> GSTIQIPYTITVNGTSQNILSSLTFNKNQNISYKDIENKVKSVLYFNRGISDIDLRLSKQA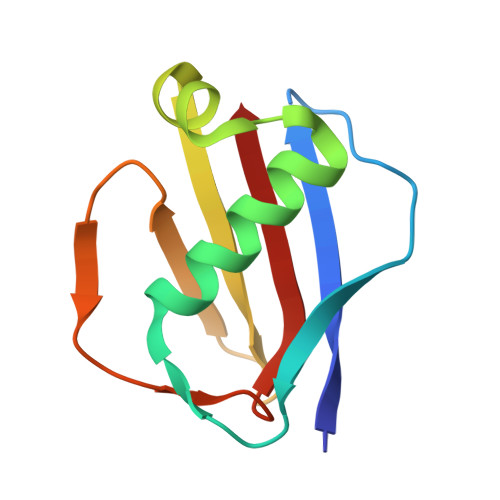EYTVHFKNGTKRVIDLKSGIYTADLINTSDIKAISVNVD> QKGPVFLKEPTNRIDFSNSTGAEIECKASGNPMPEIIWIRSDGTAVGDVPGLRQISSDGKLVFPPFRAEDYRQEVHAQVYACLARNQFGSIISRDVHVRAVVAQYYEADVNKEHVIRGNSAVIKCLIPSFVADFVEVVSWHTDEEENYFPGAEYDGKYLVLPSGELHIREVGPEDGYKSYQCRTKHRLTGETRLS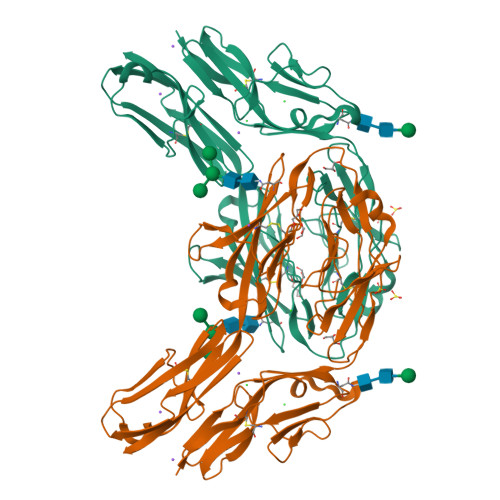ATKGRLVITEPISSSAPRTPALVQKPLELMVAHTISLLCPAQGFPAPSFRWYKFIEGTTRKQAVVLNDRVKQVSGTLIIKDAVVEDSGKYLCVVNNSVGGESVETVLTVTAPLSAKIDPPTQTVDFGRPAVFTCQYTGNPIKTVSWMKDGKAIGHSESVLRIESVKKEDKGMYQCFVRNDRESAEASAELKLG>[4x]MAPVKLYMVEVIDKKEIAANERRSRENDVTGPEITHYYQVTFRLTTDDRKDLVLNIDK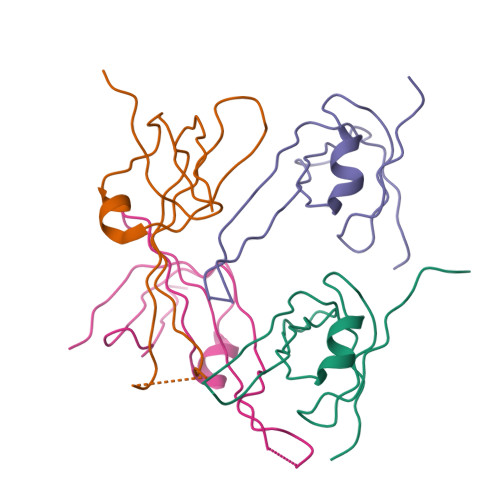SSYQNIEPEMKGRLFMQGSRFVQFETDVPIDEQKLEHHHHHH> QDNSRYTHFLTQHYDAKPQGRDDRYCEAIMRRRGLTSPCKDINTFIHGNKRSIKAICENKNGNPHRENLRISKSSFQVTTCKLHGGSPWPPC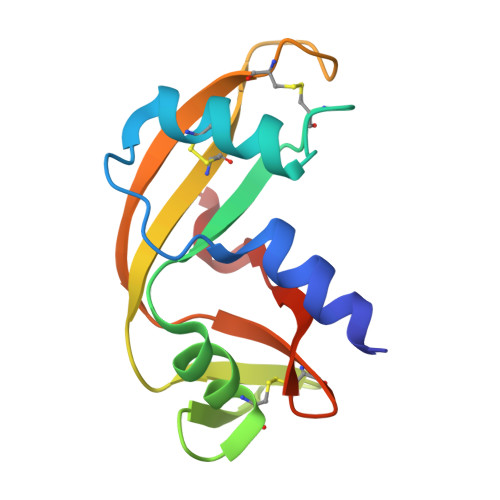QYRATAGFRNVVVACENGLPVHLDQSIFRRP> MSHSGAAIFEKVSGIIAINEDVSPAELTWRSTDGDKVHTVVLSTIDKLQATPASSEKMMLRLIGKVDESKKRKDNEGNEVVPKPQRHMFSFNNRTVMDNIKMTLQQIISRYKDADIYEEKRRREESAQHTETPMSSSSVTAGTPTPHLDTPQLNNGAPLINTAKLDDSLSKEKLLTNLKLQQSLLKGNKVLMKVFQETVINAGLPPSEFWSTRIPLLRXFALXXSQKXGPXXVXXXXXPXXXXXXXXXXNLSREKILNIFENYPIVKKAYTDNVPKNFKEPEFWARFFSSKLFRKLXXXXXXXXXXXXXXXXXXLXXXXXFXXKXXXXLLHPVKKIIXLDGNIXDDPVVRGXXXXXXXXVDILKGMNRLSEKMIMXLKXXXXXXXXXXXXXXXXXXXXXXXXXXXXXXXXXXXXXXXXRVITXIKIN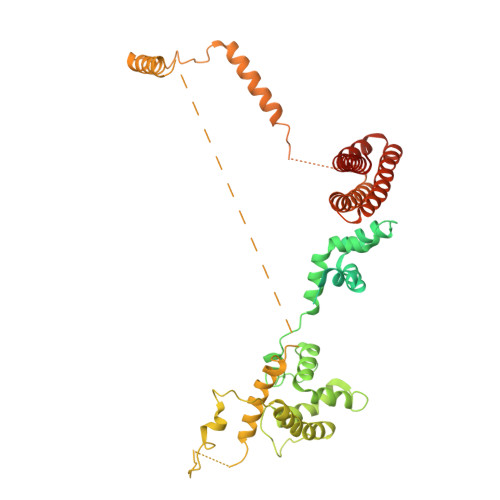AKQAXHXXXEVKSTLPIDLLESCRMLHTTCCEFLKHFAIHQKQASTVKKLYNHLKDCIEKLNELFQDVLNGDGESMSNTCTAYLKPVLNSITLATHKYDEYFNEYNNNSN The majority of mammalian poly-LacNAc is synthesized by the alternating iterative action of β1,3-N-acetylglucosaminyltransferase 2 (B3GNT2) and β1,4-galactosyltransferases. B3GNT2 is in the largest mammalian glycosyltransferase family, GT31, but little is known about the structure, substrate recognition, or catalysis by family members. Here we report the structures of human B3GNT2 in complex with UDP:Mg2+ and in complex with both UDP:Mg2+ and a glycan acceptor, lacto-N-neotetraose. The B3GNT2 structure conserves the GT-A fold and the DxD motif that coordinates a Mg2+ ion for binding the UDP-GlcNAc sugar donor.

The crystal structure of SeMet-B3GNT2 in complex with the donor analog UDP and Mg2+ (SeMet-B3GNT2:UDP:Mg2+) was solved at 1.55 Å resolution using single-wavelength anomalous diffraction. Two molecules were found in the asymmetric unit of the SeMet-B3GNT2:UDP:Mg2+ structure that were arranged as a dimer with a ∼924 Å2 interface formed between helices α4, α5 and α12 from each chain. The SeMet-B3GNT2:UDP:Mg2+ structure reveals a GT-A Rossmann-like fold comprised of eight twisted β-strands and 12 α-helical segments. The donor nucleotide sugar binds in a pocket located at the carboxy end of the GT-A fold β1 and β4 strands (secondary structure elements refer to the core GT-A fold nomenclature in Fig. S1 and Fig. 3B). There is unambiguous electron density for the Mg2+ and UDP bound in the pocket. Asp215 and Lys223 form hydrogen bonds with the uracil N3 and O2 atoms, respectively. The other side of the nucleotide sugar binding pocket is formed by Loopβ5-β6, which contains the DxD motif (Asp245-Asp246-Asp247). The last residue in the DxD motif, Asp247, acts as a ligand for coordinating the Mg2+ cation. His356 and two water molecules also interact with the metal. In the acceptor-free B3GNT2:UDP:Mg2+ and SeMet-B3GNT2:UDP:Mg2+ complexes, the Asp333 and Gly-Loop305:307 are only observed in the inactive conformation despite the fact that the latter structure was solved in a crystal form that is isomorphous to the B3GNT2:UDP:Mg2+:LNnT complex.

>[2x]GKNGKGEVIIPKEKFWKISTPPEAYWNREQEKLNRQYNPILSMLTNQTGEAGRLSNISHLNYCEPDLRVTSVVTGFNNLPDRFKDFLLYLRCRNYSLLIDQPDKCAKKPFLLLAIKSLTPHFARRQAIRESWGQESNAGNQTVVRVFLLGQTPPEDNHPDLSDMLKFESEKHQDILMWNYRDTFFNLSLKEVLFLRWVSTSCPDTEFVFKGDDDVFVNTHHILNYLNSLSKTKAKDLFIGDVIHNAGPHRDKKLKYYIPEVVYSGLYPPYAGGGGFLYSGHLALRLYHITDQVHLYPIDDVYTGMCLQKLGLVPEKHKGFRTFDIEEKNKNNICSYVDLMLVHSRKPQEMIDIWSQLQSAHLKC> MGSSHHHHHHENLYFQSDPRFPLTARDKFSLVKSWKTFSRNLESAGKEMLLKLFIEHPDMKDLFPK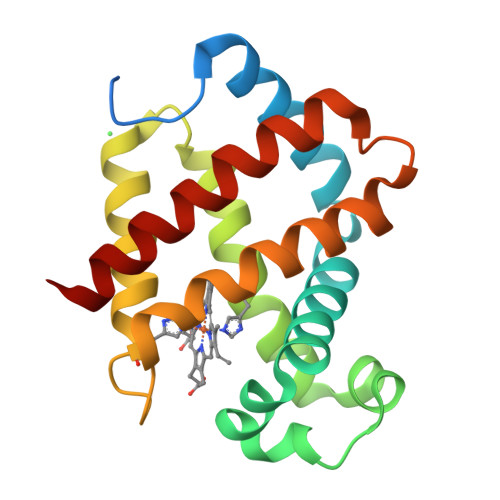FKAKTPDQLRNDESFEEAALAHITPYDQAVQDSDNVDILLTNLKRVGRQHKTVPGFQESYFERMEKCLVFALQTTLADAYTENMERIYKIWISWTTEKIREGFRE>MVSVARELTVGINGFGRIGRLVLRACMEKGVKVVAVNDPFIDPEYMVYMFKYDSTHGRYKGSVEFRNGQLVVDNHEISVYQCKEPKQIPWRAVGSPYVVESTGVYLSIQAASDHISAGAQRVVISAPSPDAPMFVMGVNENDYNPGSMNIVSNASCTTNCLAPLAKVIHERFGIVEGLMTTVHSYTATQKTVDGPSRKAWRDGRGAHQNIIPASTGAAKAVTK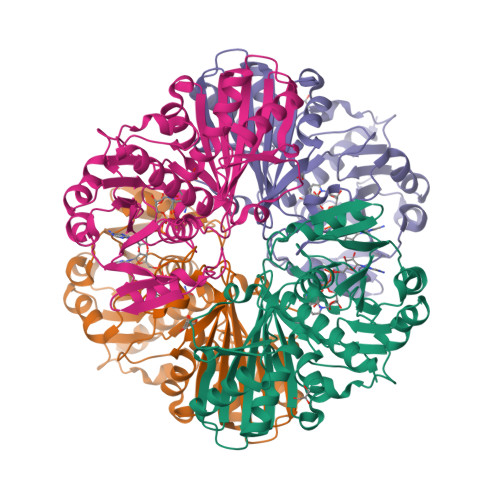VIPELKGKLTGMAFRVPTPDVSVVDLTCRLAQPAPYSAIKEAVKAAAKGPMAGILAYTEDEVVSTDFLGDTHSSIFDAKAGIALNDNFVKLISWYDNEYGYSHRVVDLLRYMFSRDAENLYFQ[2x]>METYPITVGGVTRHVPLIEPLPGRRIPLVEFLGDP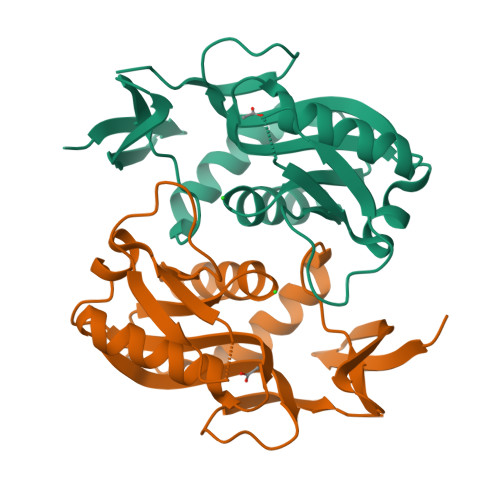EFTRAAAEALRPLVPKEAEILFTTETSPIPLTHVLAEALGLPYVVARRRRRPYMEDPIIQEVQTLTLGVGEVLWLDRRFAEKLLNQRVVLVSDVVASGETMRAMEKMVLRAGGHVVARLAVFRQGTPGLAVDTVAELPVL[5x]> MNTPKEEFQDWPIVRIAAHLPDLIVYGHFSPERPFMDYFDGVLMFVDISGFTAMTEKFSSAMYMDRGAEQLVEILNYHISAIVEKVLIFGGDILKFAGDALLALWRVERKQLKNIITVVIKCSLEIHGLFETQEWEEGLDIRVKIGLAAGHISMLVFGDETHSHFLVIGQAVDDVRLAQNMAQMNDVILSPNCWQLCDRSMIEIESVPDQRAVKVNFLKPPPNFNFDEFFTKCTTFMHYYPSGEHKNLLRLACTLKPDPELEMSLQKYVMESILKQIDNKQLQGYLSELRPVTIVFVNLMFEDQDKAEEIGPAIQDAYMHITSVLKIFQGQINKVFMFDKGCSFLCVFGFPGEKVPDELTHALECAMDIFDFCSQVHKIQTVSIGVASGIVFCGIVGHTVRHEYTVIGQKVNLAARMMMYYPGIVTCDSVTYNGSNLPAYFFKELPKKVMKGVADS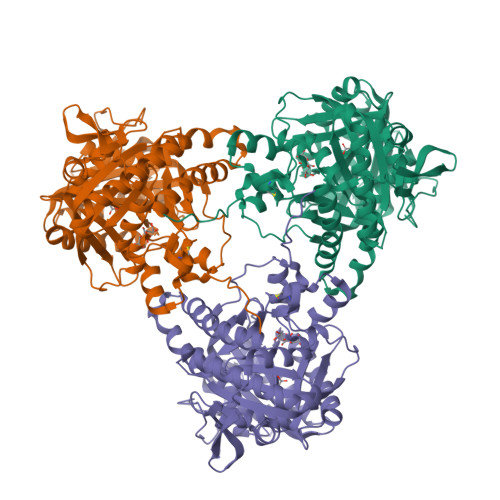GPLYQYWGRTEKVHHHHHH> MLRRSILFRMKYADLELTTRGEFPHGMKEPAFVKKL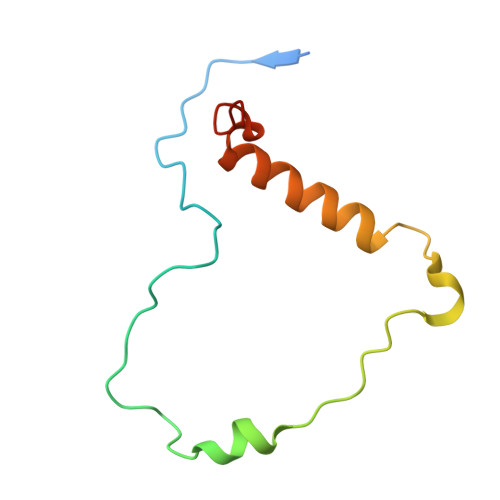DQNIPWYFSTYRSMYHWPITGDNWSDLNEAEKHHDLHMFYTLAWWKLGEGIFGVDEDS>[2x]PH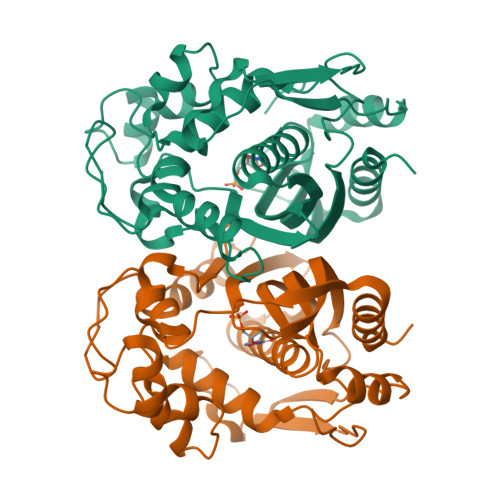EELQYLRQLREILCRGSDRLDRTGIGTLSLFGMQARYSLRDHFPLLTTKRVFWRGVVQELLWFLKGSTDSRELSRTGVKIWDKNGSREFLAGRGLAHRREGDLGPVYGFQWRHFGAAYVDADADYTGQGFDQLSYIVDLIKNNPHDRRIIMCAWNPADLSLMALPPCHLLCQFYVADGELSCQLYQRSGDMGLGVPFNIASYSLLTYMLAHVTGLRPGEFIHTLGDAHIYKTHIEPLRLQLTRTPRPFPRLEILRSVSSMEEFTPDDFRLVDYCPHPTIRMEM> FGSICAFTASRTFPNGFTVTEEFADADPIDSPPFAAADTGAGLNGDMVVWNRANILEVVVNVIPNTEGERNLAVLLDANRTGKDKSGARDVVGLVVAMPDGSKITCTNGTPIDGVLINAVAS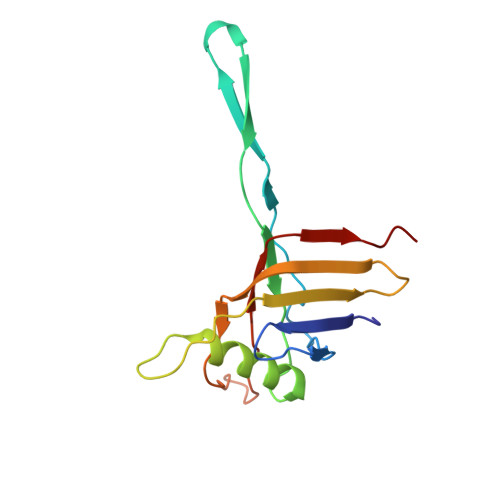VGRLKTKPYRFRFEKVIKAGTS> MDFDMIEEKKDSVIVRNVENFELKDIFDCGQCFRWHRQENG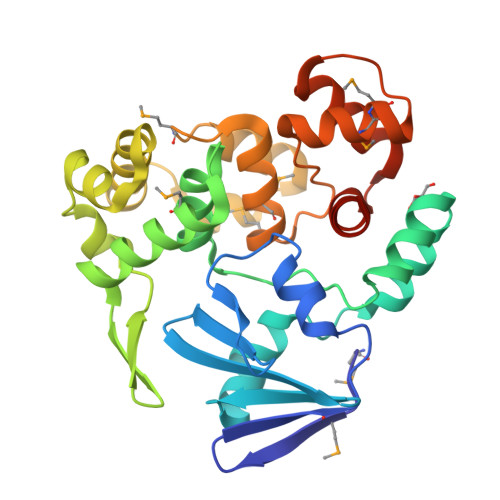NYIGIAFEKVVEVQKIGEDVVIYNINEEEFKNVWSEYFDLYRDYGEIKKELSRDPLLKKSVDFGEGIRILRQDPFEILLSFIISANNRIPMIKKCINNISEKAGKKLEYKGKIYYAFPTVDKLHEFTEKDFEECTAGFRAKYLKDTVDRIYNGELNLEYIKSLNDNECHEELKKFMGVGPKVADCIMLFSMQKYSAFPVDTWVKKAMMSLYVAPDVSLKKIRDFGREKFGSLSGFAQQYLFYYARENNIGL>[2x]SNAMTQKFDVVVIGAGPGGYVAAIKAAQLGLKTACIEKYTDAEGKLALGGTCLNVGCIPSKALLDSSWKYKEAKESFNVHGISTGEVKMDVAAMVGRKAGIVKNLTGGVATLFKANGVTSIQGHGKLLAGKKVEVTKADGTTEVIEAENVILASGSRPIDIPPAPVDQNVIVDSTGALEFQA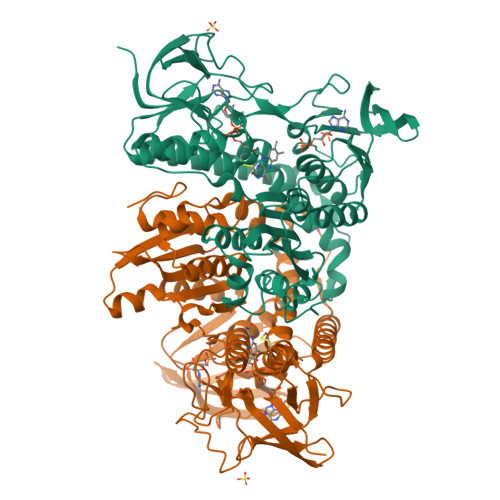VPKRLGVIGAGVIGLELGSVWARLGAEVTVLEALDTFLMAADTAVSKEAQKTLTKQGLDIKLGARVTGSKVNGNEVEVTYTNAEGEQKITFDKLIVAVGRRPVTTDLLASDSGVTIDERGYIFVDDYCATSVPGVYAIGDVVRGMMLAHKASEEGIMVVERIKGHKAQMNYDLIPSVIYTHPEIAWVGKTEQALKAEGVEVNVGTFPFAASGRAMAANDTGGFVKVIADAKTDRVLGVHVIGPSAAELVQQGAIAMEFGTSAEDLGMMVFSHPTLSEALHEAALAVNGGAIHVANRKKR> MLRRVPRVLQKGERGLYFPINHRIVDHRIAPGVTVEETDVQSRYRRELRTNFATGETRQTIAPPWSARERPTHFFSLRLPSRNSVTLRVKEMHNHLLFSHQQCAPMLVSPTKLHITLGVMTIPENSREELVKNIQQSMSETFACVQPLQLRF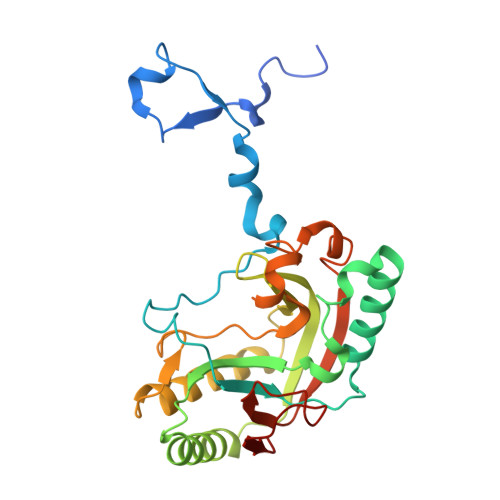RGLGTFDFGRVLFIRVVPEADFGRLERAVCDIRRRVGGVLGVDLKGNPHDSYVPHVTVAKIRPNQRQQLGDTIPQSLWADYQHHDFGDVTLSTVDLCRMKGSPDGYYHTEGAVHLS>[4x]GLEDCDFGWSPYDQHCYQAFNEQKTWDEAEKFCRAQENGAHLASIESNGEADFVSWLISQKDELADEDYVWIGLRAQNKEQQCSSEWSDGSSVSYENLIDLHTKKCGALEKLTGFRKWVNYYCEQMHAFVCKLLPY;>[4x]MGRFIFVSFGLLVVFLSLSGTGADCPSGWSSYEGHCYKPFNEPKNWADAERFCKLQPKHSHLVSFQSAEEADFVV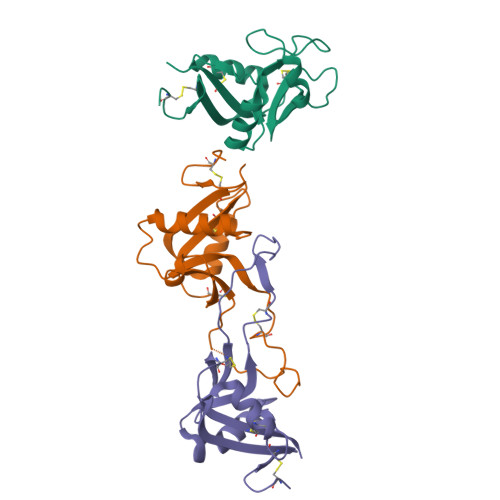KLTRPRLKANLVWMGLSNIWHGCNWQWSDGARLNYKDWQEQSECLAFRGVHTEWLNMDCSSTCSFVCKFKA;>[4x]GSGHKSSPCDTNWRYYGDSCYGFFRHNLTWEESKQYCTDMNATLLKIDNRNIVEYIKARTHLIRWVGLSRQKSNEVWKWEDGSVISENMFEFLEDGKGNMNCAYFHNGKMHPTFCENKHYLMCERKAG>MPREYEFAEKILFTEEEIRTRIKEVAKRIADDYKGKGLRPYVNPLVLISVLRGSFMFTADLCRALCDFNVPVRMEFICVSSYGEGLTSSGQVRMLLDTRHSIEGHHVLIVEDIVDTALTLNYLYHMYFTRRPASLKTVVLLDKREGRRVPFSADYVVANIPNAFVIGYGL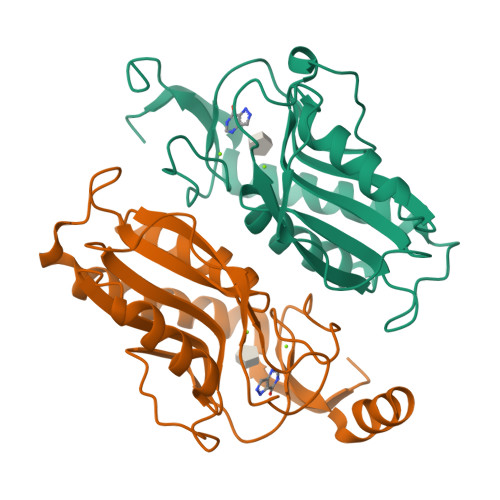DYDDTYRELRDIVVLRPEVYAEREAARQKKQRAIGSADTDRDAKREFHSKY[2x]>[8x]MKAKIRILDMFSGRYTVL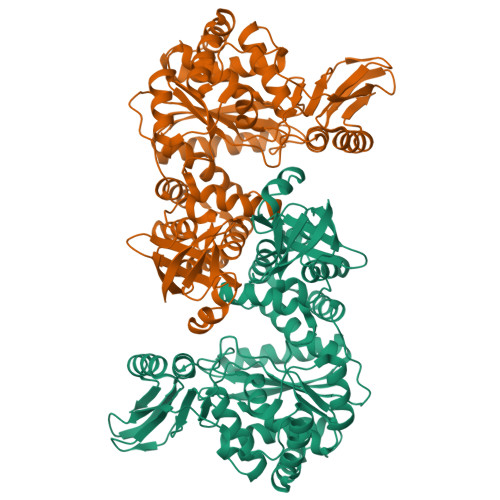INEEDAKEAKLHPDDLVKIEAGKKAVYGSVALSNLVGKGEVGISRDVLDLHNFSEGETVSVIPAGTPESVRYIKKKMHGEKLRKVEIEAIVRDIVDRKLRDIEISSFVTALEINGLDMDEIAALTIAMAETGDMLDIDRKPIMDVHSIGGVPGNKTNILVVPIVAAAGLTIPKTSSRAITSAAGTADVVEVFADVSFSLDEIKRIVEKVGACLVWGGALNLAPADDITIKAERALSIDPTGLMLASIMSKKYAMGSQYVLIDIPTGKGVKVETVEEARSLARDFIELGKRLGQYVEVAITYGGQPIGHTVGPALEAREALSALMTGKGPGSLIEKATGLAGILLEMGGVAPAGTGKKMAKEILESGKAWEKMKEIIEAQGGDPNIKPEEIPIGDKTYTFTAATSGYVTAIDNRAITAIARAAGAPEDKGAGIELYVKVGEKVKEGDPLFTIHAEHEARLDQAIVLARRTEPIRIEGNSSSVDKLAAALEHHHHHH> AHMGCVSSKSTTVLSPQTSFNEASRTSFRALPGPSQRQLEVYDQCLIGAARWPDDSSKSNTPENRAYCQSMYNSIRSAGDEISRGGITSFEELWGRATEWRLSKLQRGEPLYSAFASERTSDTDAVTPLVKPYKSVLARVVDHEDAHDEIMQDNLFGDLNVKVYRQTAYLHGNVIPLNTFRVATDTEYLRDRVAHLRTELGAKALKQHLQRYNPDRIDHTNASYLPIIKDHLNDLYRQAISSDLSQAELISLIARTHWWAASAMPDQRGSAAKAEFAARAIASAHGIELPPFRNGNVSDIEAMLSGEEEFVEKYRSLLDSDCF;> APKFGDWDENNPSSADGYTHIFNKVRDEVD

AvrB, a type III secretion system effector from the plant pathogen Pseudomonas syringae, is a member of the Fido (Fic, Doc, and AvrB) family that triggers HR in Arabidopsis plants to ward off systemic infection. Our investigations herein reveal the distinct and unexpected activity of AvrB acting as a glycosyltransferase that rhamnosylates residue T166 of Arabidopsis thaliana guardee protein RIN4. By elucidating the crystal structures of AvrB and its substrates across different enzymatic states, we provide an explanation for the specificity of substrates and delineate the step-by-step reaction mechanism executed by AvrB in the process of transferring rhamnose to RIN4. The identified biochemical activity of the avirulence protein AvrB as a rhamnosylator adds to the catalytic versatility of the Fido domain–containing protein superfamily.

Structures of AvrB + RIN4 [similar to a reported structure (19)], AvrB + RIN4 + UDP-rhamnose, AvrB + RIN4T166-Rha + UDP, and AvrBR266A + UDP together contribute to deciphering the catalytic mechanisms of AvrB as a rhamnosyltransferase. Because of its source from a plant bacterial pathogen, we hypothesized that AvrB may use UDP-rhamnose, a common plant metabolite. In the cosubstrate binding pocket, UDP-rhamnose adopts a conformation with rhamnose close to the hydroxyl group of T166 (prereaction state). UDP (free or in UDP-rhamnose) and rhamnose (in UDP-rhamnose) interact with AvrB directly and indirectly through water molecules (described in the figure legend). Contacts between UDP and AvrB: O2′-G46, α-PO4-R99, β-PO4-R266, and β-PO4-G267. Contacts between rhamnose and AvrB: O0″-T166 (RIN4), O0″-Y131, O2″-A269, O3″-D297, O4″-T166 (RIN4), and O4″-T125. The α-PO4 likely provides a driving force for priming the reaction by stabilizing the sugar moiety. dTDP-rhamnose could also be exploited by AvrB to rhamnosylate RIN4. Unlike the Fido enzyme AnkX that requires Mg2+ for catalysis, AvrB-catalyzed rhamnosylation of RIN4 does not require divalent cations. Thus, AvrB is a glycosyltransferase that uses UDP-rhamnose to rhamnosylate RIN4 on T166 in vitro.> MNSTPIEEARSLLNPSNAPTRYAERSVGPFSLAAIWFAMAIQVAIFIAAGQMTSSFQVWQVIVAIAAGCTIAVILLFFTQSAAIRWGINFTVAARMPFGIRGSLIPITLKALLSLFWFGFQTWLGALALDEITRLLTGFTNLPLWIVIFGAIQVVTTFYGITFIRWMNVFASPVLLAMGVYMVYLMLDGADVSLGEVMSMGGENPGMPFSTAIMIFVGGWIAVVVSIHDIVKECKVDPNASREGQTKADARYATAQWLGMVPASIIFGFIGAASMVLVGEWNPVIAITEVVGGVSIP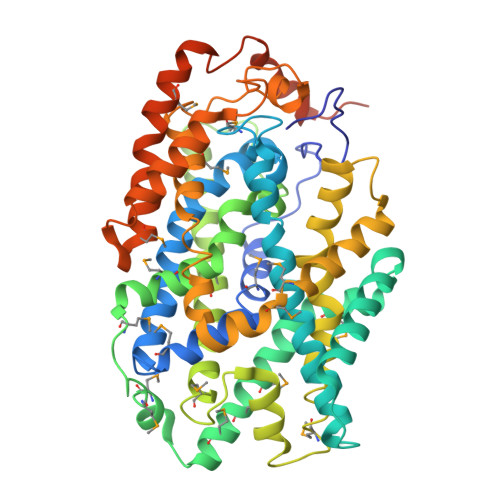MAILFQVFVLLATWSTNPAANLLSPAYTLCSTFPRVFTFKTGVIVSAVVGLLMMPWQFAGVLNTFLNLLASALGPLAGIMISDYFLVRRRRISLHDLYRTKGIYTYWRGVNWVALAVYAVALAVSFLTPDLMFVTGLIAALLLHIPAMRWVAKTFPLFSEAESRNEDYLRPIGPVAPADESATANTKEQNQPAGGRGSHHHHHH>MSAIFAERALLPEGWARNVRFEISADGVLAEIRPDANADGAERLGGAVLPGMPNLHSHAFQRAMAGLAEVAGNPNDSFWTWRELMYRMVARLSPEQIEVIACQLYIEMLKAGYTAVAEFHYVHHDLDGRSYADPAELSLRISRAASAAGIGLTLLPVLYSHAGFGGQPASEGQRRFINGSEAYLELLQRLRAPLEAAGHSLGLCFHSLRAVTPQQIATVLAAGHDDLPVHIHIAEQQKEVDDCQAWSGRRPLQWLYENVAVDQRWCLVHATHADPAEVAAMARSGAVAGLCLSTEANLGDGIFPATDFLAQGGRLGIGSDSHVSLSVVEELRWLEYGQRLRDRKRNRLYRDDQPMIGRTLYDAALAGGAQALGQPIGSLAVGRRADLLVLDGNDPYLASAEGDALLNRWLFAGGDRQVRDVMVAGRWVVRDGRHAGEERSARAFVQVLGELLD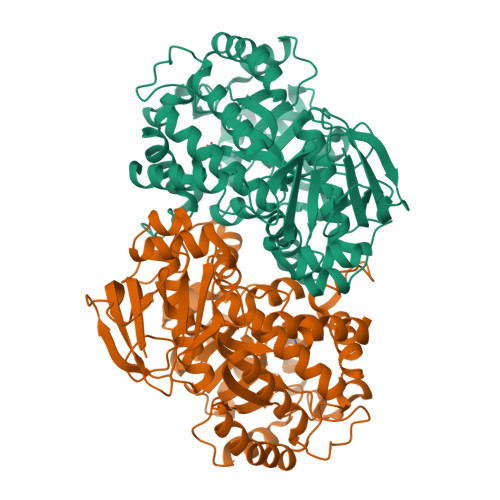[4x]> GGLEKDFLPLYFGWFLTKKSSETLRKAGQVFLEELGNHKAFKKELRHFISGDEPKEKLELVSYFGKRPPGVLHCATKFCDYGKAAGAEEYAQQEVVKRSYGKAFKLSISALFVTPKTAGAQVVLTDQELQLWPSDLDKPSASEGLPPGSRAHVTLGCAADVQPVQTGLDLLDILQQVKGGSQGEAVGELPRGKLYSLGKGRWMLSLTKKMEVKAIFTGYYG

2′,3′-cyclic nucleotide 3′-phosphodiesterase (CNPase) comprises 4% of total myelin protein in the central nervous system (CNS), being the most abundant CNS non-compact myelin protein4. CNPase consists of an N-terminal polynucleotide kinase-like domain10, a catalytic phosphodiesterase domain11, and a membrane-anchored C-terminal tail, which contains a cysteine residue that undergoes isoprenylation. The catalytic domain enables the rapid hydrolysis of nucleoside 2′,3′-cyclic phosphates to nucleoside 2′-phosphates. The CNPase catalytic site, lying in a groove between two lobes, has pseudo two-fold symmetry and contains two apposing His-X-Thr-X (X denotes a hydrophobic residue) motifs, characteristic for 2H phosphoesterases 113537.

In addition to the catalytic His mutants, near-complete catalytic inactivation is evident also in T232A, T311A, F235A, F235L, and Y168A. The inactivation by the T232A and T311A mutations was expected: threonine or serine is found in the catalytic motif in all 2H phosphoesterases, and in CNPcat, they are involved in all stages of catalysis, in achieving the correct substrate binding mode together with His230, His309, and the active-site water network.(5Z)-5-[(3-methoxyphenyl)methylidene]-2-sulfanylidene-1,3-thiazolidin-4-one | C11 H9 N O2 S2 | 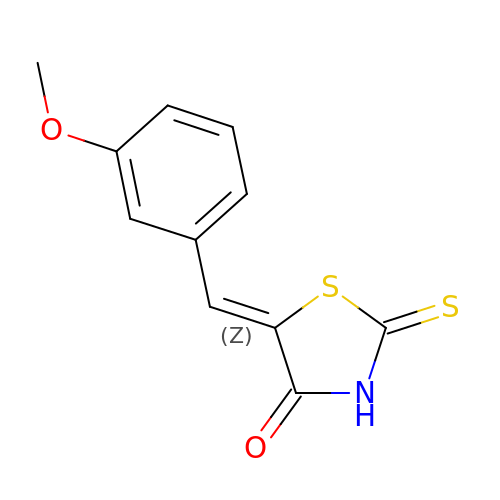ZXBRDIMYFRPBGK-TWGQIWQCSA-N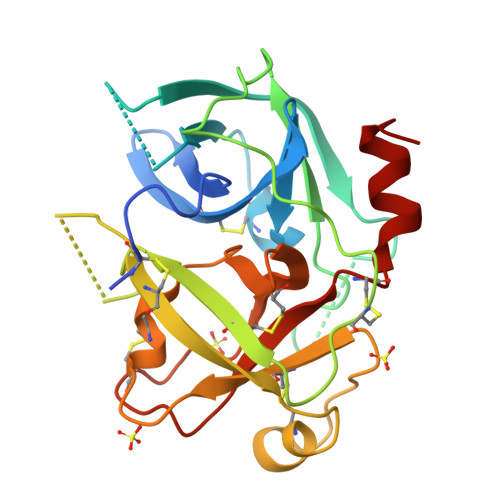>[2x]LDPEAYGSPCARGSQPWQVSLFNGLSFHCAGVLVDQSWVLTAAHCGNKPLWARVGDDHLLLLQGEQLRRTTRSVVHPKYHQGSGPILPRRTDEHDLMLLKLARPVVLGPRVRALQLPYRCAQPGDQCQVAGWGTTAARRVKYNKGLTCSSITILSPKECEVFYPGVVTNNMICAGLDRGQDPCQSDSGGPLVCDETLQGILSWGVYPCGSAQHPAVYTQICKYMSWINKVIRSN>TRLQEKEDLQELNDRLAVYIDRVRSLETENAGLRLRITESEEVVSREVSGIKAAYEAELGDARKTLDSVAKERARLQLELSKVREEFKELKARNTKKEGDLIAAQARLKDLEALLNFKEAALSTALSEKRTLEGELHDLRGQVAKLEAALGEAKKQLQDEMLRRVDAENRLQTM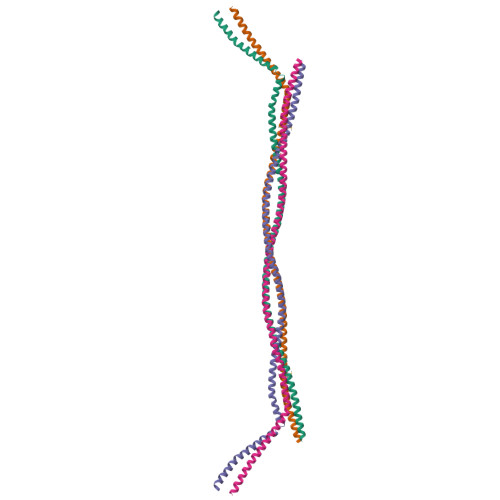KEELDFQKNIYSEELRETKRRHETRLVEIA[2x]> MSIRYESVENLLTLIKDKKIKPSDVVKDIYDAIEETDPTIKSFLALDKENAIKK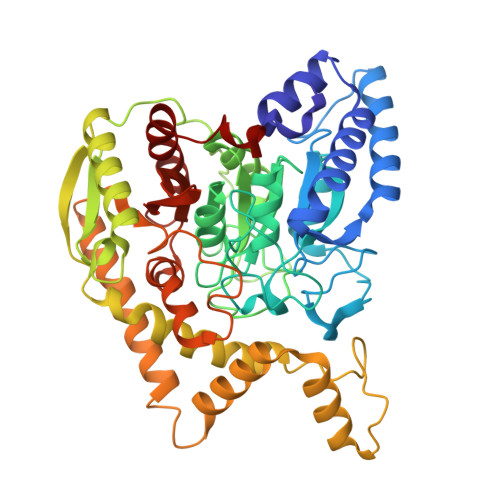AQELDELQAKDQMDGKLFGIPMGIKDNIITNGLETTCASKMLEGFVPIYESTVMEKLHKENAVLIGKLNMDEFAMGGSTETSYFKKTVNPFDHKAVPGGSSGGSAAAVAAGLVPLSLGSDTGGSIRQPAAYCGVVGMKPTYGRVSRFGLVAFASSLDQIGPLTRNVKDNAIVLEAISGADVNDSTSAPVDDVDFTSEIGKDIKGLKVALPKEYLGEGVADDVKEAVQNAVETLKSLGAVVEEVSLPNTKFGIPSYYVIASSEASSNLSRFDGIRYGYHSKEAHSLEELYKMSRSEGFGKEVKRRIFLGTFALSSGYYDAYYKKSQKVRTLIKNDFDKVFENYDVVVGPTAPTTAFNLGEEIDDPLTMYANDLLTTPVNLAGLPGISVPCGQSNGRPIGLQFIGKPFDEKTLYRVAYQYETQYNLHDVYEKL> TLKLCSPEEFTRLCREKTQEIYPIKEANGRTRKALIICNTEFKHLSLRYGANFDIIGMKGLLEDLGYDVVVKEELTAEGMESEMKDFAALS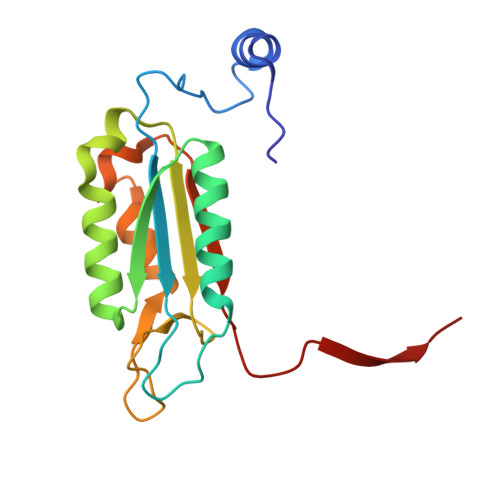EHQTSDSTFLVLMSHGTLHGICGTMHSEKTPDVLQYDTIYQIFNNCHCPGLRDKPKVIIVQAARGGNSGEMWIRES>MAMHPRKDWYELTRATNWTPSYVTEEQLFPERMSGHMGIPLEKWESYDEPYKTSYPEYVSIQREKDAGAYSVKAALERAKIYENSDPGWISTLKSHYGAIAVGEYAAVTGEGRMARFSKAPGNRNMATFGMMDELRHGQLQLFFPHEYCKKDRQFDWAWRAYHSNEWAAIAAKHFFDDIITGRDAISVAIMLTFSFETGFANMQFLGLAADAAEAGDYTFANLISSIQTDESRH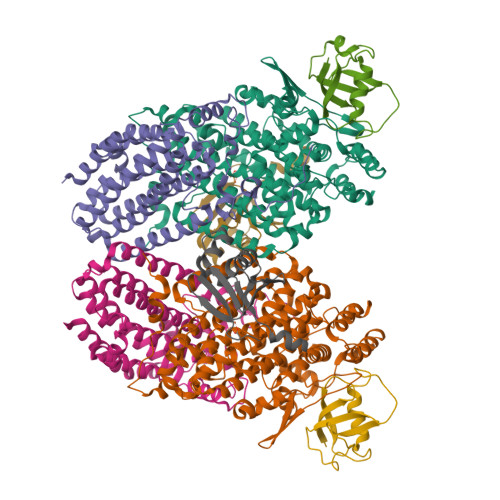AQQGGPALQLLIENGKREEAQKKVDMAIWRAWRLFAVLTGPVMDYYTPLEDRSQSFKEFMYEWIIGQFERSLIDLGLDKPWYWDLFLKDIDELHHSYHMGVWYWRTTAWWNPAAGVTPEERDWLEEKYPGWNKRWGRCWDVITENVLNDRMDLVSPETLPSVCNMSQIPLVGVPGDDWNIEVFSLEHNGRLYHFGSEVDRWVFQQDPVQYQNHMNIVDRFLAGQIQPMTLEGALKYMGFQSIEEMGKDAHDFAWADKCKPAMKKSA[2x];>[2x]MSFESKKPMRTWSHLAEMRKKPSEYDIVSRKLHYSTNNPDSPWELSPDSPMNLWYKQYRNASPLKHDNWDAFTDPDQLVYRTYNLMQDGQESYVQSLFDQFNEREHDQMVREGWEHTMARCYSPLRYLFHCLQMSSAYVQQMAPASTISNCCILQTADSLRWLTHTAYRTHELSLTYPDAGLGEHERELWEKEPGWQGLRELMEKQLTAFDWGEAFVSLNLVVKPMIVESIFKPLQQQAWENNDTLLPLLIDSQLKDAERHSRWSKALVKHALENPDNHAVIEGWIEKWRPLADRAAEAYLSMLSSDILHAQYLERSTSLRASILTV;>[2x]MSAFPVHAAFEKDFLVQLVVVDLNDSMDQVAEKVAYHCVNRRVAPREGVMRVRKHRSTELFPRDMTIAESGLNPTEVIDVVFEE;>MSTLADQALHNNNVGPIIRAGDLVEPVIETAEIDNPGKEITVEDRRAYVRIAAEGELILTRKTLEEQLGRPFNMQELEINLASFAGQIQADEDQIRFYFDKTM[2x]>MSLDYQGYLIDLDGTIYLGKEPIPAGKRFVERLQEKDLPFLFVTNNTTKSPETVAQRLANEFDIHVPASLVYTATLATIDYMKEANRGKKVFVIGEAGLIDLILEAGFEWDETNPDYVVVGLDTELSYEKVVLATLAIQKGALFIGTNPDKNIPTERGLLPGAGSVVTFVETATQTKPVYIGKPKAIIMERAIAHLGVEKEQVIMVGDNYETDIQSGIQNGIDS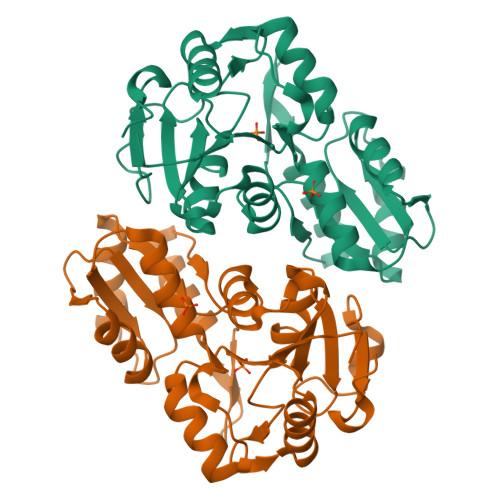LLVTSGFTPKSAVPTLPTPPTYVVDSLDEWTFEGHHHHHH[2x]>[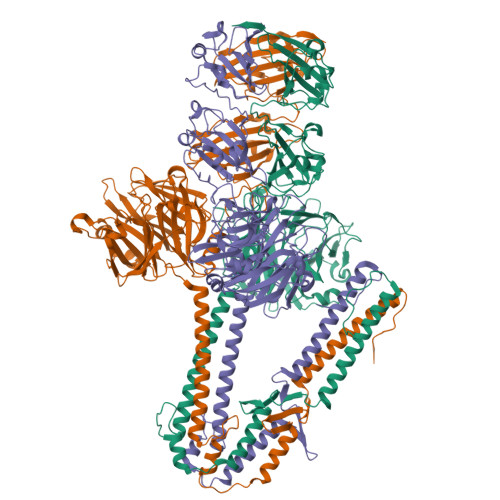3x]HHHHHHLVPRGSMSNKLITDLSRVFDYRYVDENEYNFKLISDMLTDFNFSLEYHRNKEVFAHDGEQIKYEHLNVTSNVSDFLTYLNGRFSNMVLGHNGDGINEVKDARVDNTGYGHKTLQDRLYHDYSTLDVFTKKVEKAVDEHYKEYRATEYRFEPKEQEPEFITDLSPYTNAVMQSFWVDPRTKIIYMTQARPGNHYMLSRLKPNGQFIDRLLVKNGGHGTHNAYRYIDGELWIYSAVLDSNKNNKFVRFQYRTGEITYGNEMQDVMPNIFNDRYTSAIYNPVENLMIFRREYKPTERQLKNSLNFVEVRSADDIDKGIDKVLYQMDIPMEYTSDTQPMQGITYDAGILYWYTGDSNTANPNYLQGFDIKTKELLFKRRIDIGGVNNNFKGDFQEAEGLDMYYDLETGRKALLIGVTIGPGNNRHHSIYSIGQRGVNQFLKNIAPQVSMTDSGGRVKPLPIQNPAYLSDITEVGHYYIYTQDTQNALDFPLPKAFRDAGWFLDVLPGHYNGALRQVLTRNSTGRNMLKFERVIDIFNKKNNGAWNFCPQNAGYWEHIPKSITKLSDLKIVGLDFYITTEESNRFTDFPKDFKGIAGWILEVKSNTPGNTTQVLRRNNFPSAHQFLVRNFGTGGVGKWSLFEGKVVE>[2x]GSHMDKNEKLIEEYKYRLQKLQNDEMIWTKERQSLLEKMNNTENY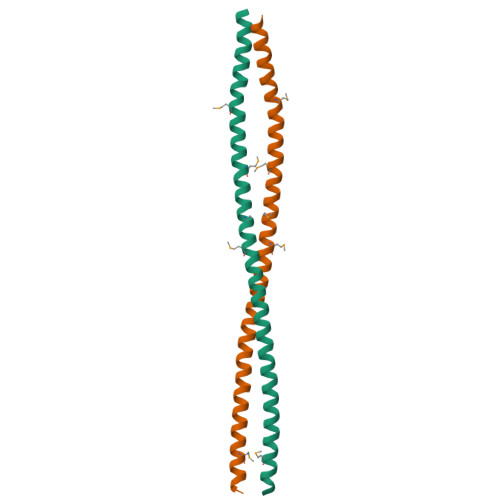KIEMIKENEMLREQLKEAQSKLNEKNIQLRSKEIDVNKLSDRVLSLENELRNMEIELDRNKKRND> MTENILRKSDEEIQKEITARVKALESMLIEQGILTTSMIDRMAEIYENEVGPHLGAKVVVKAWTDPEFKKRLLADGTEACKELGIGGLQGEDMMWVENTDEVHHVVVCTLCDCYPWPVLGLPPNWF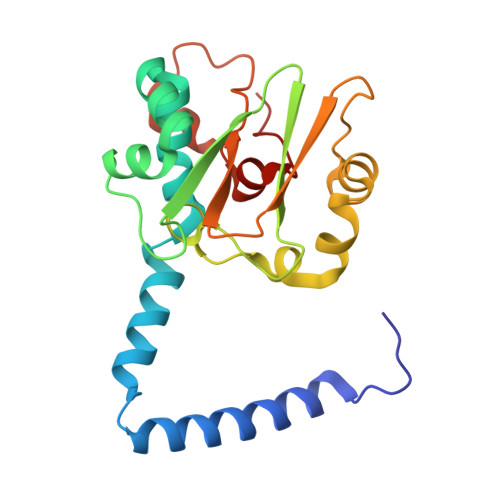KEPQYRSRVVREPRQLLKEEFGFEVPPSKEIKVWDSSSEMRFVVLPQRPAGTDGWSEEELATLVTRESMIGVEPAKAV The fusobacterial trimeric autotransporter adhesin (TAA) CbpF binds to CEACAM1 on immune cells, resulting in downregulation of their activity against tumors colonized by F. nucleatum. In contrast to Fap2, CbpF is a homotrimeric type Vc autotransporter protein, in which all three protomers together form a trimeric passenger domain that remains exposed on the cell surface after expression, and a C-terminal β-barrel domain that serves as a membrane anchor. The ECD of CEACAM1 comprises an N-terminal, membrane-distal immunoglobulin variable region-like (IgV-like) domain and three membrane-proximal immunoglobulin constant region-like (IgC2-like) domains IgC2-like A1, IgC2-like B, and IgC2-like A2. CbpF binds to CEACAM1 via a protruding loop (D142–Y149) and via H92 on the respective adjacent protomer chain.

We therefore formed the complex of nanodisc-reconstituted CbpF and CEACAM1-ECD (residues 35–428, ACRO Biosystems) and removed excess of CEACAM1 by preparative size exclusion chromatography (SEC). We then vitrified the SEC fraction corresponding to the main peak and resolved the structure of the complex to 2.7 Å, applying C3 symmetry. The structure revealed a heterohexameric complex in which one CEACAM1 is bound per CbpF protomer, with the N-terminal IgV-like domain of CEACAM1 and the region around the β roll protruding loop of CbpF forming the interface. Each CEACAM1 protrudes perpendicularly from the central CbpF trimer and sits atop the β roll protruding loop of CbpF. Four residues of the eight-residue long loop 142–149, i.e., E142, N144, Q146, and Q148, form H-bonds with side chains of T90, Q78 [Q44 in mature chain (11)], and Y68 of CEACAM1. In addition, there are two further H-bonds three β strands “above” in the stack that are formed between H92 and N99 of CbpF and the backbone of S127 and D128 of CEACAM1. Importantly, H92 originates from the neighboring CbpF protomer, and both together form one CEACAM1 interface. Instead, a tight interface is formed exclusively by the peptide moieties predominantly via H-bonds, whereas only two hydrophobic surface-exposed residues (F63 and L129 in CEACAM1) are buried in the complex. The rest of the CEACAM1 side of the interface appears slightly negatively charged, whereas at the CbpF side of the interface, positive charges dominate. Our CbpF/CEACAM1 complex structure shows that CEACAM1-F63 is in close proximity to H92 and F143, which probably form aromatic stacking interactions.

>[3x]MKKTAIAIAVALAGFATVAQASAAPVIKAGTATDSTEAGVDNVANGVKSSAFGYDNKAIEKESSAFGTGNRATGEFSSAFGFHNIASKIHSSAFGSNNAADGVNSSAFGFKNTVSGFNSSAFGSQYQVTGNFSGAFGMGEFNGQYQYKNEGNNSYMIGNKNKIASGSDDNFILGNNVHIGGGINNSVALGNNSTVSASNTVSVGSSTLKRKIVNVGDGAISANSSDAVTGRQLYSGNGIDTAAWQNKLNVTRKNDYKDANDIDVNKWKAKLGVGSGGGGGAPVDAYTKSEADNKFANKTDLNDYTKKDDYKDANGIDVDKWKAKLGTGAGTADIENLRNEVNEKIDDVKDEVRTVGSLSAALAGLHPMQYDPKAPVQVMAALGHYRDKQSVAVGASYYFNDRFMMSTGIALSGEKRTKTMANVGFTLKLGKGSGVTYDETPQYVVQNEVKRLTVENQELKERVRNLEEKLNMLLKNKRSSAWSHPQFEK;>QLTTESMPFNVAEGKEVLLLVHNLPQQLFGYSWYKGERVDGNRQIVGYAIGTQQATPGPANSGRETIYPNASLLIQNVTQNDTGFYTLQVIKSDLVNEEATGQFHVYPELPKPSISSNNSNPVEDKDAVAFTCEPETQDTTYLWWINNQSLPVSPRLQLSNGNRTLTLLSVTRNDTGPYECEIQNPVSANRSDPVTLNVTYGPDTPTISPSDTYYRPGANLSLSCYAASNPPAQYSWLINGTFQQSTQELFIPNITVNNSGSYTCHANNSVTGCNRTTVKTIIVTELSPVVAKPQIKASKTTVTGDKDSVNLTCSTNDTGISIRWFFKNQSLPSSERMKLSQGNTTLSINPVKREDAGTYWCEVFNPISKNQSDPIMLNVNYNALPQENGLSPGHHHHHH[3x]Here, we present biochemical and structural evidence that POA inhibits Mtb PanD in a competitive fashion and that it binds with a high degree of complementarity to the active site of the enzyme. PanD is a proenzyme and in the structure, we observed the processed active enzyme after cleavage between Gly24 and Ser25, and modification of Ser25 to a pyruvoyl group (Pyr25). The active protein consists of a β chain (Met1-Gly24) and an α chain (Pyr25 to ILE115). Our results show that resistance to PZA in PanD mutants primarily comes from alterations in two loops covering the active site that have subtle, but significant effects on the affinity and residence time of POA on the enzyme rather than from directly affecting POA binding interactions.

Crystals of Mtb PanD were produced using the hanging-drop vapor diffusion method. The crystal structures of apo Mtb PanD and the Mtb PanD:POA complex were solved using molecular replacement and both structures were refined to 2.7 Å resolution. The first 115 residues were clearly visible in the electron density map, while the last 24 residues could not be built due to the flexibility at the C-terminus.

>[6x]MLRTMLKSKIHRATVTCADLHYVG;>[6x]XVTIDADLMDAADLLEGEQVTIVDIDNGARLVTYAITGERGSGVIGINGAAAHLVHPGDLVILIAYATMDDARARTYQPRIVFVDAYNKPIDMGHDPAFVPENAGELLDPRLGVGLEHHHHHH> MGKTFTVPIVEVTSSFNPATFQSLLIPRDNRPLEVGLLRKVKELLAEVDARTLARHVTKVDCLVARILGVTKEMQTLMGVRWGMELLT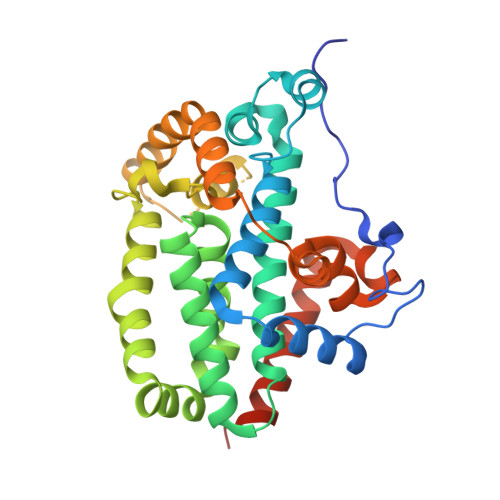LPHGRQLRLDLLERFHTMSIMLAVDILGSTGSAEERAALLHKTIQLAAELRGTMGNMFSFAAVMGALDMAQISRLEQTWVTLRQRHTEGAILYEKKLKPFLKSLNEGKEGPPLSNTTFPHVLPLITLLESDSAPPEGPEPWGSTEHGVEVVLAHLEAARTVAHHGGLYHTNAEVKLQGFQARPELLEVFSTEFQMRLLWGSQGASSSQARRYEKFDKVLTALSHKLEPAVRSSELLEHHHHHH> MGRVADTIARGPSNSEQIPALTAVETGHTSQVDPSDTMQTRHVHNYHSRSESSIENFLCRSACVIYIKYSSAESNNLKRYAEWVINTRQVAQLRRKMEMFTYIRCDMELTFVITSHQEMSTATNSDVPVQTHQIMYVPPGGPVPTSVNDYVWQTSTNPSIFWTEGNAPPRMSIPFMSIGNAYTMFYDGWSNFSRDGIYGYNSLNNMGTIYARHVNDSSPGGLTSTIRIYFKPKHVKAYVPRPPRLCQYKKAKNVNFDVEAVTTERASLVTT;> SDRVRSITLGNSTITTQECANVVVGYGVWPDYLSDEEATAEDQPTQPDVATCRFYTLNSVKWEMQSAGWWWKFPDALSEMGLFGQNMQYHYLGRSGYTIHVQCNASKFHQGCLLVVCVPEAEMGCTNAENAPTYGDLCGGETAKQFEQNAVTGETAVQTAVCNAGMGVGVGNL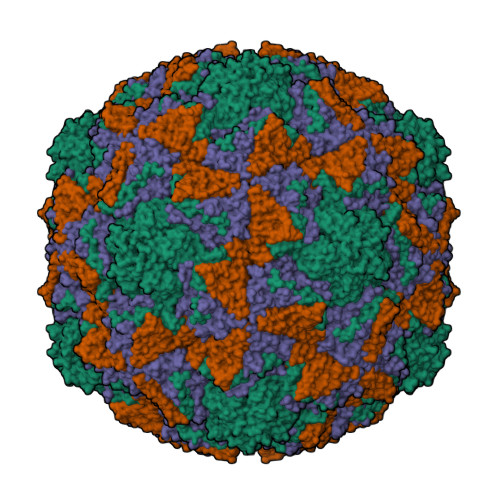TIYPHQWINLRTNNSATIVMPYINSVPMDNMFRHNNFTLMIIPFAPLDYVTGASSYIPITVTVAPMSAEYNGLRLAGHQ;> GLPTMLTPGSTQFLTSDDFQSPSAMPQFDVTPEMNIPGQVRNLMEIAEVDSVVPINNLQANLKTMEAYRVQVRSTDEMGGQIFGFPLQPGASSVLQRTLLGEILNYYTHWSGSLKLTFVFCGSAMATGKFLLAYSPPGAGAPDSRKNAMLGTHVIWDVGLQSSCVLCVPWISQTHYRYVVDDKYTASGFISCWYQTNVIVPAEAQKSCYIMCFVSACNDFSVRMLRDTQFIKQDTFYQ;> MGAQVSTQKTGAHETSLSASGNSIIHYTNINYYKDAASNSANRQDFTQDPSKFTEPVKDVMIKSLPALN> GSDLTVSLIPVSGLKAGKNAPSAKIA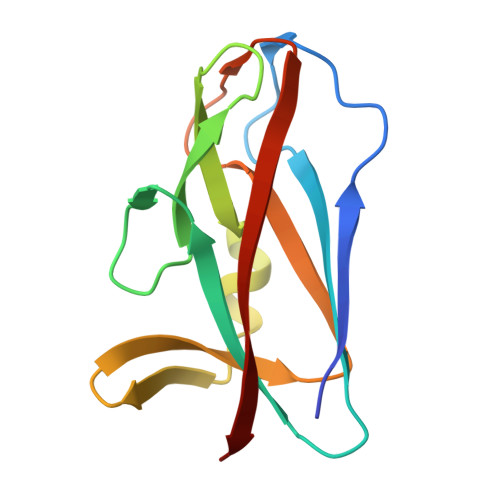KLVVNSTTLKEFGVRGISNNVVDSTGTAWRVAGKNTGKEIGVGLSSDSLRRSDSTEKWNGVNWMTFNSNDTLDIVLTGPAQNVTADTYPITLDVVGYQP Methanothermococcus thermolithotrophicus is the only known methanogen that grows on sulfate as its sole sulfur source, uniquely uniting methanogenesis and sulfate reduction. Here we use physiological, biochemical and structural analyses to provide a snapshot of the complete sulfate reduction pathway of this methanogenic archaeon. M. thermolithotrophicus activates SO42− by conventional ATPS and APSK, but transforms it further by uncanonical enzymes.

No genes encoding for a canonical PAPS reductase (route 1b) or sulfo-transferase (route 1c) were found in the M. thermolithotrophicus genome. However, genes annotated as dissimilatory APS reductase (α and β subunit, APSR) are present and co-occur with the previously described genes. To gain further molecular insights into the unconventional APS-reductase-like enzyme from M. thermolithotrophicus, the enzyme was crystallized under anaerobic conditions. The structure was solved by a single-wavelength anomalous dispersion experiment measured at the Fe K-edge and refined to 1.45 Å resolution. The complex organizes as an α2β2 heterotetramer, with the same assembly as dissimilatory APS reductases. It is, however, drastically different from characterized single-domain assimilatory APS/PAPS reductases, which are thioredoxin/glutathione-dependent. The residues coordinating APS, invariable in the dissimilatory family, differ in M. thermolithotrophicus and might provoke a switch of specificity from APS to PAPS. Despite a short soak with PAP, the putative substrate pocket contains only solvent, and we used the AfAPSR to artificially model PAPS in the active site of the enzyme. The different substitutions mainly carried by loop 104–123 would accommodate the additional 3′-phosphate group by salt-bridge interactions and hydrogen bonds. In APS reductases, however, a conserved glutamine (α145 in A. fulgidus) would clash with this phosphate group. Taking together the enzyme rates and the structural analysis, we propose that M. thermolithotrophicus harbours a unique class of PAPS reductase (MtPAPSR) used to convert PAPS into SO32− and PAP.

>[2x]MDVKKIFTDILIIGGGAAGCQAAIRAKEIDKNLDVLIVEKANIIRSGCLAAGVNAINAYLNEGETPESYVEYVKKESSGLIREDLTYTIGKRLNKMAKKLEEYGLPIQKDENGRYVARGKRSIKINGESIKPILAEATLKAGVKVLNNTIATNYILKDETVCGAYAFSIKENKFYVIMAKAVICTTGGASGIYKPNNPGAARHKMWYSPFNTGAGFAMGLRAGAEMTTFEMRFIALRVKDVISPTGTIAQGVKVSQINALGEKYMEKYENNTTPMRLYATLIENLEGRGPCYLDTRGISDEDVQKLKEAYLSMSPGIILKWKDEKINPKNTPIEICGSEPYIVGGHGQAGYWVDINRKTTLEGLYAAGDVVGGSPKKYVTGCMAEGEIAVEAAIEYIKSMENDIEIDEQEIAKEIDRVFYPLNNKKGEFSPDEIEERMQKVMDEYAGGISSYYRVNESKLLIARELLKAIEEDLSKIKVRNRYELMKYHEVVDRILVARAVVEHLLYRKETRWKCYQERVDYPEIDDNWFKFINSKYNSQTNDIEIIEREYEKFNPVINNDHSSGHHHHHH;>[2x]MTIRIIEEICIGCGLCTKVCPGNLLYQREDGKSEIMDKRDCWDCAACVKECPVNAIEMYLQPEIGGRGSTLKAKKTDDSIVWIITDNNGEEEVIEVKNKKTFDM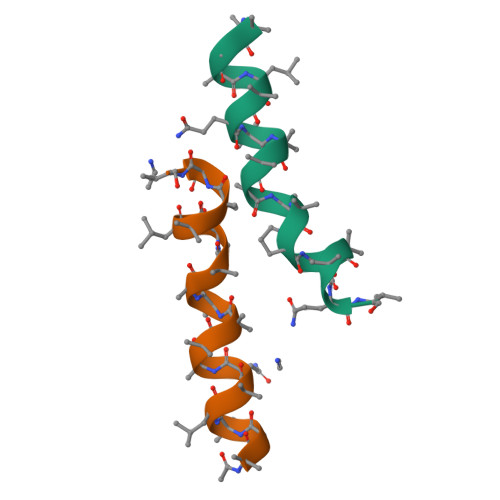>[2x]XAGALAQAAAAAAPLAAQX The structure of the N-sites of HIV-1 RT and HBV Pol are considered to be quite similar, as the amino acid sequences that form the N-sites (referred to as motifs A, B, C, D, and E) are moderately conserved in both. In our previous studies, we examined various combinations of amino acid substitutions in motifs A–E and found that the HBV-RT-associated 3MB mutant comprising Q151M in motif B and Y115F/F116Y in motif A is useful as a surrogate for structurally studying HBV RT since HIV-1 harboring RT3MB turned out to be highly sensitive against typical anti-HBV NAs, ETV, and 3TC. E-CFCP is a 4′-modified and fluoromethylenated NA that exhibits potent antiviral activity against both wild-type and drug-resistant HBVs but less potent against human immunodeficiency virus type-1 (HIV-1). The present study aimed to elucidate the mechanism of potent antiviral activity of E-CFCP against wild-type and drug-resistant HBV using HIV-1 with HBV-associated mutations in RT.

We also determined the structures of HIV-1 RT4M complexed with DNA:ETV-TP/dGTP at 2.32 and 2.30 Å resolutions, respectively, as reference models for comparison. In contrast, the bound ETV-TP/dGTP are well ordered and superimposed with each other with an RMSD of 0.2–0.3 Å, and their average B-values were similar to those of polypeptide chains and DNA (~ 60 Å2), suggesting that the bound ETV-TP/dGTP is rather static within the N-site. Due to the concavity formed by the Met184 sidechain, the hydrophobic pocket is expanded toward the side of Met184; the interatomic distances between Met184 CG and Ala114 CB are 8.0–8.8 Å and 6.0–6.5 Å in the E-CFCP-TP and dNTP complexes, respectively. Superimposition of the bound E-CFCP-TP, ETV-TP, and dGTP in HIV-1 RT3MB/4M highlights the deviated binding of the cyclopentyl moiety of E-CFCP-TP; the cyclopentyl moiety is shifted approximately 0.6 Å toward Met151 and skewed by approximately 10°. We anticipated that comparing the structures of RT3MB and RT4M would help us understand the structural impact of L74V on the N-site, enabling us to predict the compatibility of E-CFCP-TP binding to the HBV RT N-site.

>[2x]MVPISPIETVPVKLKPGMDGPKVKQWPLTEEKIKALVEICTEMEKEGKISKIGPENPYNTPVFAIKKKDSTKWRKVVDFRELNKRTQDFWEVQLGIPHPAGLKQKKSVTVLDVGDAFYSVPLDKDFRKYTAFTIPSINNETPGIRYQYNVLPMGWKGSPAIFQSSMTKILEPFRKQNPDIVIYQYMDDLYVGSDLEIGQHRTKIEELRQHLLRWGFTTPDKKHQKEPPFLWMGYELHPDKWTVQPIVLPEKDSWTVNDIQKLVGKLNWASQIYAGIKVRQLSKLLRGTKALTEVVPLTEEAELELAENREILKEPVHGVYYDPSKDLIAEIQKQGQGQWTYQIYQEPFKNLKTGKYARMKGAHTNDVKQLTEAVQKIATESIVIWGKTPKFKLPIQKETWEAWWTEYWQATWIPEWEFVNTPPLVKLWYQLEKEPIIGAETFYVDGAANRETKLGKAGYVTDRGRQKVVPLTDTTNQKTELQAIHLALQDSGLEVNIVTDSQYALGIIQAQPDKSESELVSQIIEQLIKKEKVYLAWVPAHKGIGGNEQVDKLVSAG;>[2x]MAHHHHHHALEVLFQGPISPIETVPVKLKPGMDGPKVKQWPLTEEKIKALVEICTEMEKEGKISKIGPENPYNTPVFAIKKKDSTKWRKLVDFRELNKRTQDFWEVQLGIPHPAGLKQKKSVTVLDVGDAYFSVPLDKDFRKYTAFTIPSINNETPGIRYQYNVLPQGWKGSPAIFQSSMTKILEPFRKQNPDIVIYQYMDDLYVGSDLEIGQHRTKIEELRQHLLRWGFTTPDKKHQKEPPFLWMGYELHPDKWTVQPIVLPEKDSWTVNDIQKLVGKLNWASQIYAGIKVRQLSKLLRGTKALTEVVPLTEEAELELAENREILKEPVHGVYYDPSKDLIAEIQKQGQGQWTYQIYQEPFKNLKTGKYARMKGAHTNDVKQLTEAVQKIATESIVIWGKTPKFKLPIQKETWEAWWTEYWQATWIPEWEFVNTPPLVKLWYQ> 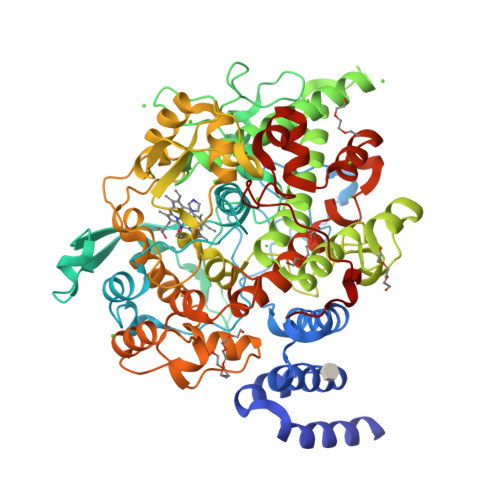MRGSHHHHHHGSMKVITSLISSILLKFIHKDFHEIYARMSLLDRFLLLIVHGVDKMVPWHKLPVFLGLTYLEVRRHLHQQYNLLNVGQTPTGIRFDPANYPYRTADGKFNDPFNEGVGSQNSFFGRNCPPVDQKSKLRRPDPMVVATKLLGRKKFIDTGKQFNMIAASWIQFMIHDWIDHLEDTHQIELVAPKEVASKCPLSSFRFLKTKEVPTGFFEIKTGSQNIRTPWWDSSVIYGSNSKTLDRVRTYKDGKLKISEETGLLLHDEDGLAISGDIRNSWAGVSALQALFIKEHNAVCDALKDEDDDLEDEDLYRYARLVTSAVVAKIHTIDWTVQLLKTDTLLAGMRANWYGLLGKKFKDSFGHAGSSILGGVVGMKKPQNHGVPYSLTEDFTSVYRMHSLLPDQLHILDIDDVPGTNKSLPLIQEISMRDLIGRKGEETMSHIGFTKLMVSMGHQASGALELMNYPMWLRDIVPHDPNGQARPDHVDLAALEIYRDRERSVPRYNEFRRSMFMIPITKWEDLTEDEEAIEVLDDVYDGDVEELDLLVGLMAEKKIKGFAISETAFYIFLIMATRRLEADRFFTSDFNETIYTKKGLEWVNTTESLKDVIDRHYPDMTDKWMNSESAFSVWDSPPLTKNPIPLYLRIPSR>[36x]DPFTMAAYTIVKEEESPIAPHRLFKALVLERHQVLVKAQPHVFKSGEIIEGDGGVGTVTKITFVDGHPLTYMLHKFDEIDAANFYCKYTLFEGDVLRDNIEK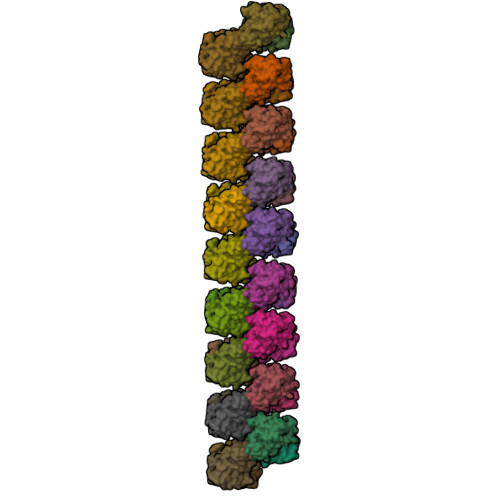VVYEVKLEAVGGGSKGKITVTYHPKPGCTVNEEEVKIGEKKAYEFYKQVEEYLAANPEVFA> GSHMYPIATNLKVSNNQLDSYLPIRNKNNNIDWQIVTGLVLSYAVKYKIDTYSLEQFREDC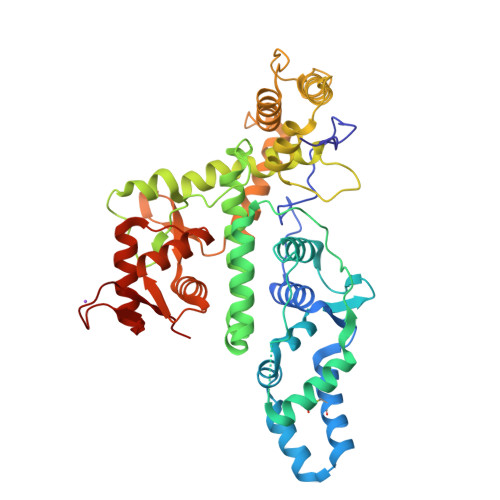KTHLQILIDEPAFLSVLERMYFSSQDIFRVSPLFLLFHAQFDGEKISAGSTADKRLGTLFANLMRDFSLNNPIQDKLNFIEKEMLNKLNKKLIRLGEGPFAKEQPYLPYLVTCFQSDLAFLAEHPQYLLQELTNTLRLYAFSWCAQLALNLDNWQDGEPQSKSLFFILDTEKASSERDKIKLFGYKWFARQSEKLFPVLSALEVLQVKGEEKRPLWQVYQDCLGYSDTSNRVLNELNNYIQKFISKEERDLPERDRATNLEDAFKQLLSVAVEQFQGKKTERAAVNRKYINELESQICTDFIQVRGRAGKVLVLNQDRLLLLTNLTVGKNKKLRLHELLRGFEQRGFYLDNQSTQMLVAFYERMGNVERMSDSGDAVYVRKTV>GSNNSETPAPGPDSLLALAFPSDPQVSPDGKQVAFVLAQISEEDPAKPDKDFARPRYRSGLWLSEGGAARPLTHAETGRGDSAPRWSPDGQNLAFVRSAGEVKAALMLLPLKGGEARRVTHFKNGVSGPQWSPDGRFIAFTTTADTEDKRDERGEARVLTRPVYRANGADWLPERPAALWLYDVEADKLREWYAPEIGIGALSWWPDSRGVLIVQSEDEWQASQWRQDVYDLPLPTADAPAAPQKLLDWNSAAHGLAPHPDGQRFALIGRPAGKGNTEHAHLYLIENGQHRRLDTGHDHPVGDAVGGDCHVGAFPEGPRWLDGDTLLFSSTVRGSVGLFTAHIGGGVKAYDHDPQGVISAFTANEHGVALIRESATRFPEVELNGQRVTDLHARFPFPVREPQRVTFETELGEGEGWVLLPEGEQKVPALLNIHGGPHTDYGHGFTHEFQLMAARGYGVCYSNPRGSVGYGQAWVDAIYGRWGTVDADDLLN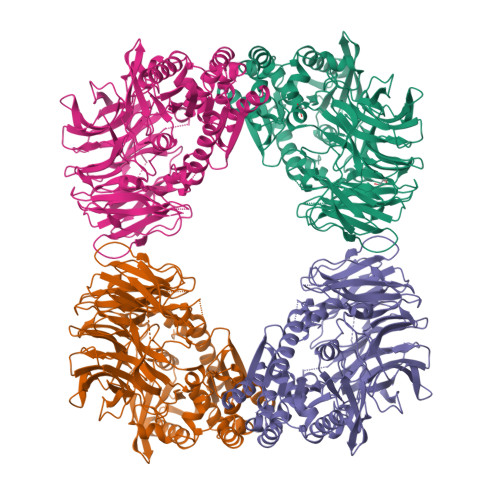FFDRCLEAVPRLDAAKTAVMGGAYGGFMTNWITGHTTRFQAAITDRCISNLISFGGTSDIGLRFWDDELGLDFSRRADALKLWDLSPLQYVENVKTPTLIVHSVLDHRCPVEQAEQWYAALHKHQVPVRFVRFPEENHELSRSGRPDRRLTRLNEYFAWLERWL[4x]>MTTSQKHRDFVAEPMGEKPVGSLAGIGEVLGKKLEERGFDKAYVVLGQFLVLKKDEDLFREWLKDTCGAN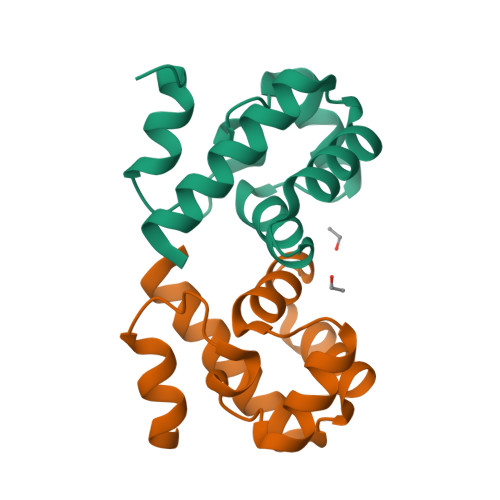AKQSRDCFGCLREWCDAFL[2x]>[6x]AAAEEARNKAHVAPGELDEYYGFWSGGHQGEVRVLGVPSMRELMRIPVFNVDSATGWGITNESKEILGGDQQYLNGDCHHPHISMTDGRYDGKYLFINDKANTRVARIRLDIMKTDKITHIPNVQAIHGLRLQKVPKTNYVFCNAEFVIPQPNDGTDFSLDNSYTMFTAIDAETMDVAWQVIVDGNLDNTDADYTGKYATSTCYNSERAVDLAGTMRNDRDWVVVFNVERIAAAVKAGNFKTIGDS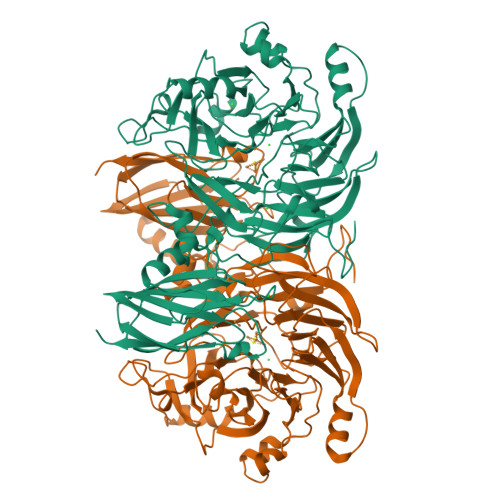KVPVVDGRGESEFTRYIPVPKNPHGLNTSPDGKYFIANGKLSPTVSVIAIDKLDDLFEDKIELRDTIVAEPELGLGPLHTTFDGRGNAYTTLFIDSQVCKWNIADAIKHYNGDRVNYIRQKLDVQYQPGHNHASLTESRDADGKWLVVLSKFSKDRFLPVGPLHPENDQLIDISGEEMKLVHDGPTYAEPHDCILVRRDQIKTKKIYERNDPYFASCRAQAEKDGVTLESDNKVIRDGNKVRVYMTSVAPQYGMTDFKVKEGDEVTVYITNLDMVEDVTHGFCMVNHGVSMEISPQQTASVTFTAGKPGVYWYYCNWFCHALHMEMVGRMLVEAA>MTEPLPRIQHYEDLGLGLFIHWGLYSQMAVGEWTELIHHRNQHDYEQLIKTFTAAQFDAKKIAHAAKAVGAKYIVLTTKHHEGFFLYDTKGLSDFDVMHAPARRDLIAEFVAACREEDLLPFFYMATYDWHTPLYDDDFPAYLTYLQKSVEVLCRNYGPVGGFWFDGNWNKKDADWHLPELYGMIRHYQPNAIIVNNTGLKNRGQVSDPEIDVVTYQRRTPDEIYHGAPNEKYVAGEISITLNQHWGIAANDLNYKSPAEVIETVAHARHIGANILVNIGLTGTGAIPAAAQTYMHLLGRWTAMAAPVLYKGRPVPVTSAHGTRDFVLHTSKHDFLCILDLQVVGNDNVVLGGEGVNPRSFVGIGQPIQRIHWLDNDEVLSFTQDLDKKVLTVDAT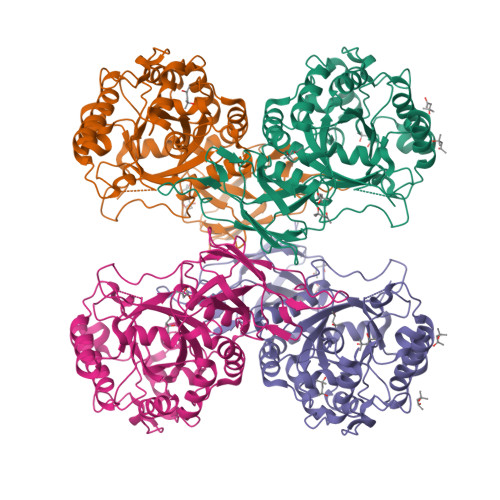GYPYGSDWVVRIAQIDYE[6x]> SVHVPGPHAMTIQELVDYVNARQKQGIYEEYEDIRRENPVGTFHCSMSPGNLEKNRYGDVPCLDQTRVKLTKRSGHTQTDYINASFMDGYKQKNAYIGTQG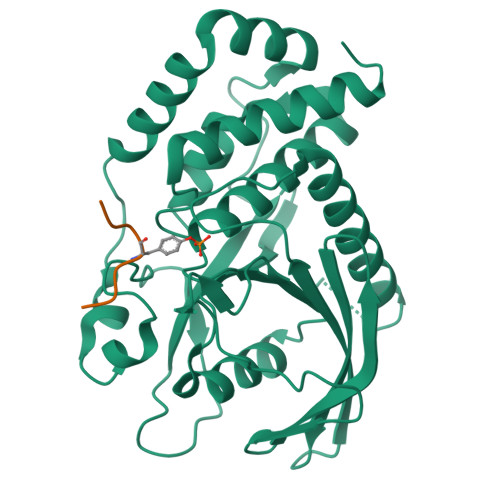PLENTYRDFWLMVWEQKVLVIVMTTRFEEGGRRKCGQYWPLEKDSRIRFGFLTVTNLGVENMNHYKKTTLEIHNTEERQKRQVTHFQFLSWPAYGVPSSAASLIDFLRVVRNQQSLAVSNMGARSKGQCPEPPIVVHASAGIGRTGTFCSLDICLAQLEELGTLNVFQTVSRMRTQRAFSIQTPEQYYFCYKAILEFAEKEGMVSS;> EVSLYTFDK> MSLKALINGTIYTSFNPLKKVSGLVISHGKVIYAGDSEVAKKIVELSGGEIVDLKGKYVMPAFFDSHLHLDELGMSLEMVDLRGAKSIEELIQRLKRGKGRIIFGFGWDQDELGEWPTRKELNAIDKPVFIYRKCFHVAVANDKMLELLNLTPSKDFDEDTGIIKEKSLEEARKVINERVLTVEDYVYYIKRAQEHLLDLGVKSVSFMSVNEKALRALFYLEREGKLSINVFAYVTPEVLDKLESIGLGRFQGNRLTIAGVKLFTDGSLGARTALLSKPYSDDPSTSGQLVMEREELIRITEKARSLGLDVAIHAIGDKALDVALDVFETTGFPGRIEHASLVRDDQLERVKNLKVRLSVQPHFIISDW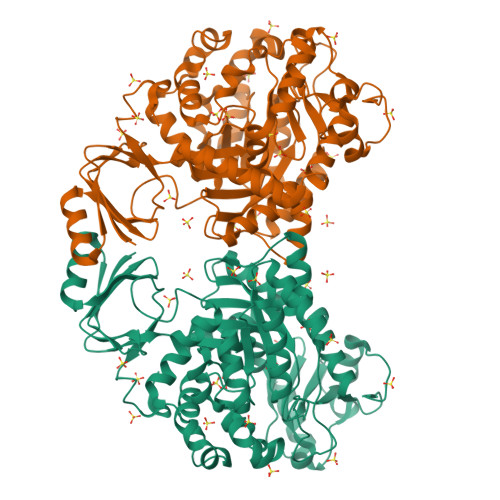WIVERVGEERVKWVYRFKDLMKVAELGFSTDSPIEPADPWLTVDAAVNRGKGKVKLYELTKDQALDIKDALHSYTYGSARVSLASDIGKLEPGFKAEYIILDRDPLVVKEGHHHHHH>[36x]XVQSKIGSLDNITHX

Functional tau is most abundant in neuronal axons where it binds to microtubules, assists microtubule assembly, and is essential for the structural integrity of neurons and for axonal transport. Here, we identify a new amyloidogenic segment, PAM4 (Polymorphic AMyloid segment in repeat 4), encompassing residues 350–362 of R4, and show that it self-assembles into amyloid fibrils. Cryo-EM revealed that PAM4 fibrils are highly polymorphic, and, remarkably, that the polymorphs formed by this segment in isolation recapitulate the conformations that PAM4 adopts in polymorphs from different human tauopathies. In all cases, the folds share a C-terminal β-strand (residues 358–362) but differ in the way they orientate the N-terminus about an intermediary GS-bend (residues 355–356).

To perform a deeper analysis of the amyloidogenic properties of the identified PAM4 region, we next synthesised a high purity (>99%) peptide corresponding to this segment (matching residues 350–362) and characterised its ability to assemble into amyloid fibrils in more detail. Specifically, we were able to identify 2D-classes containing potential two (65%), three (28%) and four (10%) protofilament polymorphs assembled from conserved core folds. The structure of the two-protofilament morphology (PAM4 Type 1) was determined at 2.6 Å resolution, with a helical twist of 359.32° and rise of 4.86 Å corresponding to a crossover of 125 nm. Each protofilament contained six PAM4 subunits, giving a total of twelve subunits per layer of the fibril with each protofilament comprising a head-to-tail ring of PAM4 peptides. The lower abundance, larger fibril morphologies of the PAM4 peptide fibrils could not be resolved to high resolution but appeared to contain the same protofilament building blocks as PAM4 Type 1 with increasing assembly sizes. All four of the PAM4 fibril structures are inferred to be left-handed from the resolution of the cryoEM maps, as well as from cryo-electron tomography (cryoET) reconstructions of Type 1 fibrils. Interestingly, the folds were interchangeable within the different fibril types, with Type 1 contaning FoldA and B, Type 2 fibrils containing FoldB, C and D, and Type 3 and Type 4 fibrils containing FoldC and D. In the FoldA-FoldB building block (seen in PAM4 Type 1 fibrils), the FoldA subunits are similar to FoldB but bend further around the GS region to cap the end of the adjacent peptide chain. FoldB PAM4, which has a flipped N-terminal compared to the previous fold, perfectly matches the 4R PSP-derived tau fibril cores and shows a C-terminal mismatch to the 3R PiD tau polymorph.>MRKTKTEALKTKEHLMLAALETFYRKGIARTSLNEIAQAAGVTRDALYWHFKNKEDLFDALFQRICDDIENCIAQDAADAEGGSWTVFRHTLLHFFERLQSNDIHYKFHNILFLKCEHTEQNAAVIA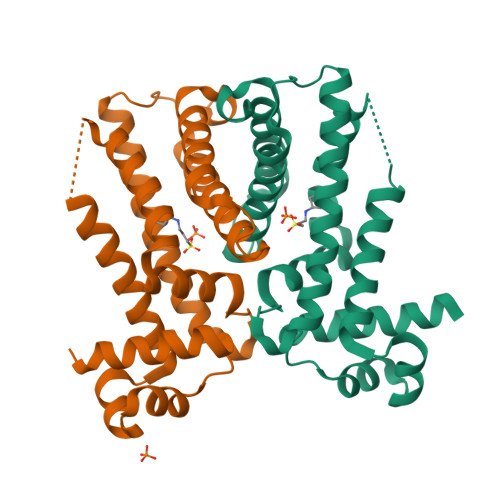IARKHQAIWREKITAVLTEAVENQDLADDLDKETAVIFIKSTLDGLIWRWFSSGESFDLGKTAPRIIGIMMDNLENHPCLRRK[4x]> MRGSHHHHHHGSKYSELADLYRRLEKTTLKTLKTKFVADFLKKTPDELLEVVPYLILGKVFPDWDERELGVGEKLLIKAVSMATGVPEKEIENSIKDTGDLGESVALALKKRKQKSFFSQPLTIKRVYSTFVKVAEASGEGSQDRKMKYLANLFMDAQPEEGKYIARTVLGTMRTGVAEGILRDAIAEAFRVKPELVERAYMLTSDFGYVAKVAKLEGNEGLSKVSIQIGKPIRPMLAQNAASVKEALIEMGGEAAFEIKYDGARVQVHRDGDRVIIYSRRLENVTRSIPEIVEAVKASLKPSK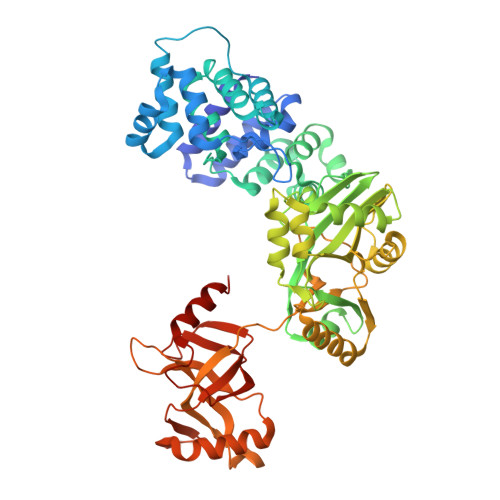VIVEGELVAVGENGRPRPFQYVLRRFRRKYNIDEMIEKIPLELNLFDILYVDGESLIDTEFVERRKRLEESVEESEKIKIAEQLVTKKVEEAEAFYKRALELGHEGLMAKRLDSVYEPGNRGKKWLKIKPTMENLDLVIIGAEWGEGRRAHLLGSFLVAAYDPDSGEFLPVGKVGSGFTDEDLVEFTKMLKPLILREEGKFVEIEPKVVIEVTYQEIQKSPKYRSGFALRFPRYVALREDKSPEEADTIERIAQLYELQEKFKAKR2-(methylamino)-1,7-dihydro-8H-imidazo[4,5-g]quinazolin-8-one | C10 H9 N5 O | 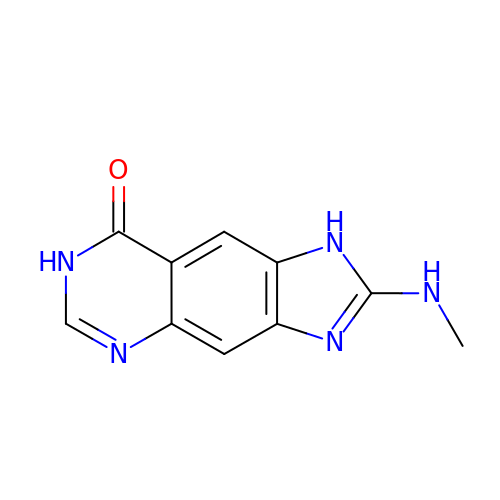DGRUEIDKEKQZFU-UHFFFAOYSA-N>GSAYQDYLARSRVGEGLALAASAR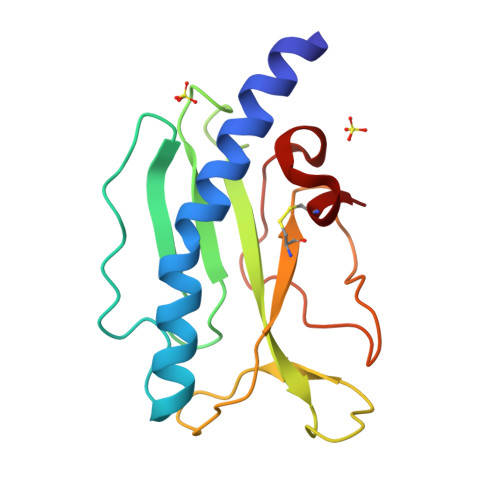LAVAENAASGNGFSGGYVSPPATRNVESIRIDDDTGQIAIAFTARVAAAGANTLVLVPSVPDQADTPTARVALSKGVIQAGTITWECFAGDKASSSLPAPGAGPMPTDAPTLAGKLAPPECRA[2x]>MWVLLRSGYPLRILLPLRGEWMGRRGLPRNLAPGPPRRRYRKETLQALDMPVLPVTATEIRQYLRGHGIPFQDGHSCLRALSPFAESSQLKGQTGVTTSFSLFIDKTTGHFLCMTSLAEGSWEDFQASVEGRGDGAREGFLLSKAPEFEDSEEVRRIWNRAIPLWELPDQEEVQLADTMFGLTKVTDDTLKRFSVRYLRPARSLVFPWFSPGGSGLRGLKLLEAKCQGDGVSYEETTIPRPSAYHNLFGLPLISRRDAEVVLTSRELDSLALNQSTGLPTLTLPRGTTCLPPALLPYLEQFRRIVFWLGDDLRSLEAAKLFARKLNPKRCFLVRPGDQQPRPLEALNGGFNLSRILRTALPAWHKSIVSFRQLREEVLGELSNVEQAAGLRWSRFPDLNRILKGHRKGELTVFTGPTGSGKTTFISEYALDLCSQGVNTLWGSFEISNVRLARVMLTQFAEGRLEDQLDKYDHWADRFEDLPLYFMTFHGQQSIRTVIDTMQHAVYVYDICHVIIDNLQFMMGHEQLSTDRIAAQDYIIGVFRKFATDNNCHVTLVIHPRKEDDDKELQTASIFGSAKASQEADNVLILQDRKLVTGPGKRYLQVSKNRFDGDVGVFPLEFNKNSLTFSIPPKNKARLKKIKDDT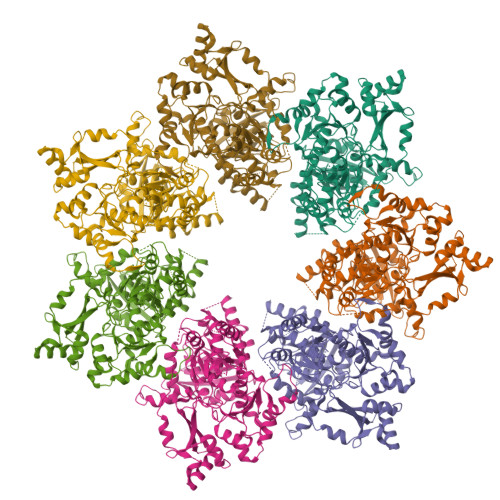GPVAKKPSSGKKGATTQNSEICSGQAPTPDQPDTSKRSKAAALEHHHHHH[7x]>[4x]GSHMAAELDSLLGQEKERFQVLPGRDKMLYVAAQNERDTLWARQVLARGDYDKNARVINENEENKRISIWLDTYYPQLAYYRIHFD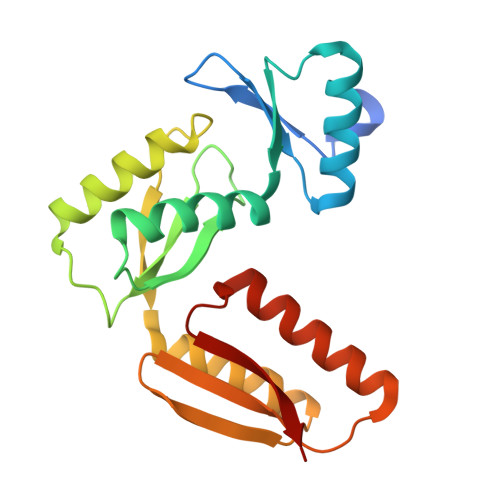EPRKPVFWLSRQRNTMSKKELEVLSQKLRALMPYADSVNITLMDDVTAAGQAEAGLKQQALPYSRRNHKGGVTFVIQGALDDVEILRARQFVDSYYRTWGGRYVQFAIELK> MTQVASPVVQARYSPVELSAALGLFPPTDEQAAVIAAPPGPLVVIAGAGAGKTETMAARVVWLVANGFATPSQVLGLTFTRKAAGQLLRRVRTRLARLAGAGLAPGSGASDESATVSTYHAFAGTLLREHGLLLPVEPDTRLLSETELWQLAYDVVCAHPGHLDTEKTPAAVTAMVLRLSGALAEHLVDTDQLRXXXXXXXXXXXXXXXXXXXXXXXXXXXLLRMLATQTERTELVPLIDALHQRMRAEKVMDFGMQMAAAARLAARFPQVGEQLRQRFRVVLLDEYQDTGHAQRIALSSLFGGGADDGLALTAVGDPIQSIYGWRGASATNLPRFTTDFPYSDGTPAPTLELRTXXXXXXXXXXXXXXXXXXXXXXXXXXXXXXXXXXXXXXTIRCALLNNVAAERDWVADHLARAYHGAIGRGEAAPTAAVLVRRNADAAPMAEALTARGVPVEVVGVAGLLAVPEVADLVAMLRLIADPTAGSAVMRILTGPRWRFGARDIAALWRRAVELDDRPKGELGTADIVAQAAPDADTACVADAICDPGDAERYSPAGYERIVALGRELTMLRAHLGHPLPELVAEVRRVLGLDAEARAARPVAAGWAGTENLDRFSDLVSDFAGHAGASVSALLAYLDAAVEVENGLAPA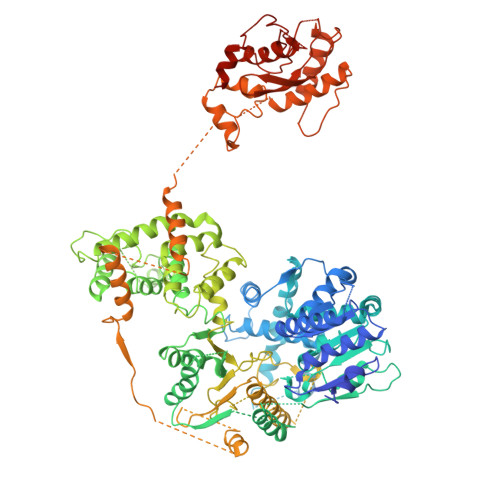ELTVSHDRVQILTVHAAKGLEWQVVAVPHLSARVFPSTTQARTWLTDASDLPPLLRGDRATESEIGVPVLDTSDIYDRKILSDKISDHKKSLDQRRVDEERRLLYVAITRAEDTLLLSGHHWGATESKPRGPSEFLCELKTILEEATAAGTPCGEIEHWAPDPAPGETNPLRDQVVEALWPPVASADDHVHRGAQLVAAAMAGEVSAEADQEGWAADVDALLAERERPXXXXXXXXXXXXXXXXXXXXXXXXXXXXXXXXXXXXXXXXXHALLGTTFHEWVQRYFHAERLFDLDDLPGAVDSDSGRAVEESLAELQDAFVKSPWAARTPVEVEVPFDMVLGETVVRGRIDAVFAEPDGTTMVLAWKTGDPPETPEAKEHAAVQLAVYRLAWAAMRGCPPESVRAAFHYVRSGXXXXXXXXXXXXXXXXXLAAAPTETAEEADRIT> VDEQPLENYLDMEYFGTIGIGTPAQDFTVVFDTGSSNLWVPSVYCSSLACTNHNRFNPEDSSTYQSTSETVSITYGTGSMTGILGYDTVQVGGISDTNQIFGLSETEPGSFLYYAPFDGILGLAYPSISSSGATPVFDNIWNQGLVSQDLFSVYLSADDQSGSVVIFGGIDSSYYTGSLNWVPVTVEGYWQITVDSITMNGEAIACAEGCQAIV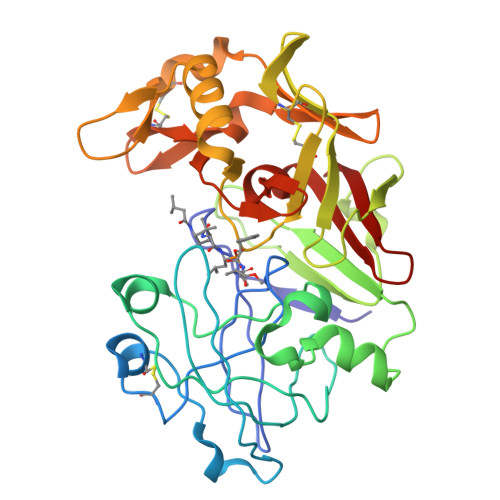DTGTSLLTGPTSPIANIQSDIGASENSDGDMVVSCSAISSLPDIVFTINGVQYPVPPSAYILQSEGSCISGFQGMNLPTESGELWILGDVFIRQYFTVFDRANNQVGLAPVA> MSVNYAAGLSPYADKGKCGLPEIFDPPEELERKVWELARLVWQSSSVVFHTGAGISTASGIPDFRGPHGVWTMEERGLAPKFDTTFESARPTQTHMALVQLERVGLLRFLVSQNVDGLHVRSGFPRDKLAELHGNMFVEECAKCKTQYVRDTVVGTMGLKATGRLCTVAKARGLRACRGELRDTILDWEDSLPDRDLALADEASRNADLSITLGTSLQIRPSGNLPLATKRRGGRLVIVNLQPTKHDRHADLRIHGYVDEVMTRLMKHLGLEIPAWDGPRVLERALPPLPRPPTPKLEPKEESPTRING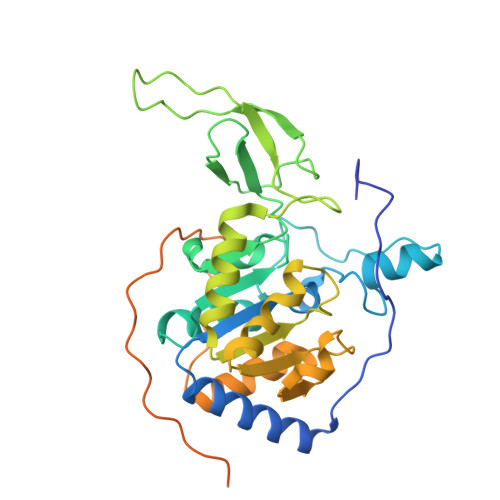SIPAGPKQEPCAQHNGSEPASPKRERPTSPAPHRPPKRVKAKAVPS3-(dimethylamino)-~{N}-[4-[4-(4-fluorophenyl)-5-(1~{H}-pyrrolo[2,3-b]pyridin-4-yl)imidazol-1-yl]cyclohexyl]propane-1-sulfonamide | C27 H33 F 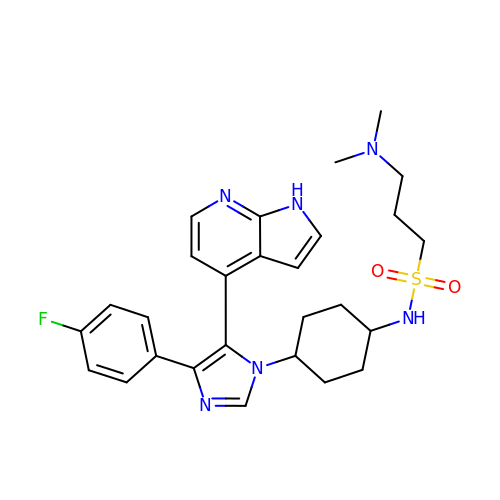N6 O2 S | MGIRTYSYARWCQY-SZPZYZBQSA-N>[2x]MRGSHHHHHHGSASFLKKTMPFKTTIEGTVNGHYFKCTGKGEGNPFEGTQEMKIEVIEGGPLPFAFHILSTSC;>[2x]MYGSKTFIKYVSGIPDYFK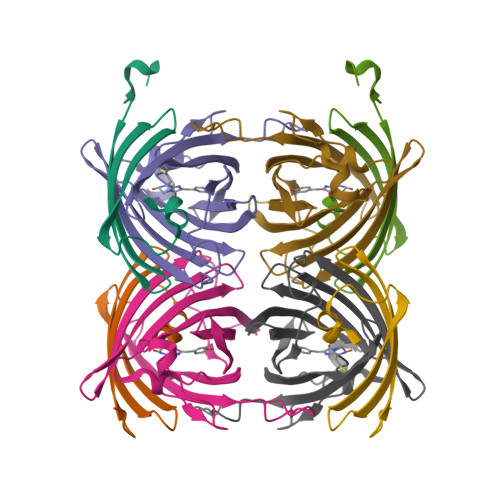QSFPEGFTWERTTTYEDGGFLTAHQDTSLDGDCLVYKVKILGNNFPADGPVMQNKAGRWEPSTEIVYEVDGVLRGQSLMALKCPGGRHLTCHLHTTYRSKKPASALKMPGFHFEDHRIEIMEEVEKGKCYKQYEAAVGRYCDAAPSKLGHN By administering enzyme drugs called L-asparaginases, which act to quickly deplete Asn in the blood, this drug specifically impacts ALL cells, starving them to death while leaving normal cells largely intact. WoA, like most bacterial Type II L-asparaginases, is a tetramer built by a dimer-of-dimer with 330 residues per protomer. In our structures we observe that the overall fold of each protomer follows the general two-domain fold of bacterial type II L-asparaginases. We sought to clarify this question and to further explain the substrate discrimination, if there is any, between the two forms, by solving the crystal structures of both variants in complex with either the product Asp or L-glutamic acid (Glu).

For WoA-P121, soaking the crystal briefly in Asp solution was sufficient in closing the loop. In sharp contrast, the structure of WoA-S121 crystals soaked in the same Asp solution, despite showing clear electron density for the Asp molecule, adopted the open loop conformation. Thus it is logical to conclude that the efficiency of active loop closing on Asn for the WoA-P121 and WoA-S121 variants would be comparable. However, as previously mentioned, soaking a WoA-P121 crystal briefly in an Asp solution was sufficient to close the N-terminal flexible loop (closed loop in pink), while multiple attempts to soak WoA-S121 crystals for many days or even co-crystallization of the WoA-S121 protein with Asp still resulted in the same Asp-bound open structure (open loop in wheat). An identical Asp binding mode was also observed between the WoA-P121 + Asp and WoA-S121 + Asp structures, despite the former having the closed, and the latter the open, N-terminal loop conformation. Thus, ambiguity exists, where on the one hand kinetic studies detect no difference between the WoA-S121 and WoA-P121 variants in their ability to hydrolyse Asn, and on the other hand, crystallographic studies show the binding of the product Asp can close the loop if the amino acid at the 121st position is a proline but not if it is a serine. When the substrate Asn is in the active site, hydrogen bonds between the substrate’s amide and the hydroxyl moieties of both Thr14 and Thr93 tether the N-terminal loop to the closed conformation. In contrast, when the product Asp is in the active site, the hydrogen network between the ligand and Thr14 is broken, hindering loop closure. In contrast, when serine replaces Pro121, a major stabilizing factor for Tyr27 is lost and it can no longer compensate for the lack of bonding between the ligand and Thr14, resulting in the WoA-S121 + Asp structure adopting the open conformation. To our knowledge, the WoA-S121 + Asp, WoA-S121 + Glu and WoA-P121 + Glu structures reported in this study represent the first L-asparaginase structures caught in its fully inactive/open state in the presence of product ligands, while the WoA-P121 + Asp structure is the first closed/active state of WoA reported so far.

>[4x]MAKPQVTILATGGTIAGSGESSVKSSYSAGAVTVDKLLAAVPAINDLATIKGEQISSIGSQEMTGKVWLKLAKRVNELLAQKETEAVIITHGTDTMEETAFFLNLTVKSQKPVVLVGAMRSGSSMSADGPMNLYNAVNVAINKASTNKGVVIVMNDEIHAAREATKLNTTAVNAFASPNTGKIGTVYYGKVEYFTQSVRPHTLASEFDISKIEELPRVDILYAHPDDTDVLVNAALQAGAKGIIHAGMGNGNPFPLTQNALEKAAKSGVVVARSSRVGSGSTTQEAEVDDKKLGFVATESLNPQKARVLLMLALTKTSDREAIQKIFSTY> GESGKKEIVVAATKTPHAEILKEAEPLLKEKGYTLKVKVLSDYKMYNKALADKEVDANYFQHIPYLEQEMKENTDYKLVNAGAVHLEPF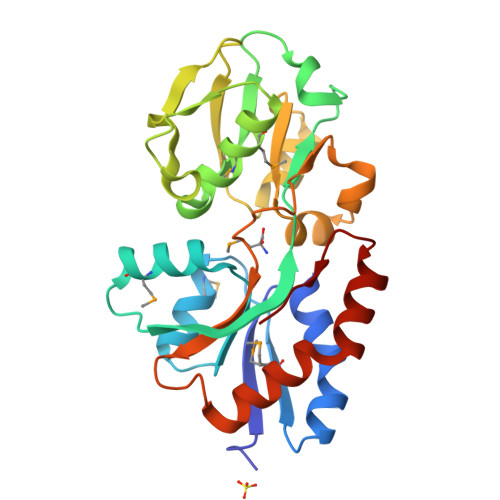GIYSKTYKSLKDLPDGATIILTNNVAEQGRMLAMLENAGLITLDSKVETVDATLKDIKKNPKNLEFKKVAPELTAKAYENKEGDAVFINVNYAIQNKLNPKKDAIEVESTKNNPYANIIAVRKGEEDSAKIKALMEVLHSKKIKDFIEKKYDGAVLPVSE>MGDDLLLKLLELLVEQARVSAEFARRQGDEKMLEEVARKAEEVARKAESIARKARKEGNLELALKALEILVRAAHVLAEIARERG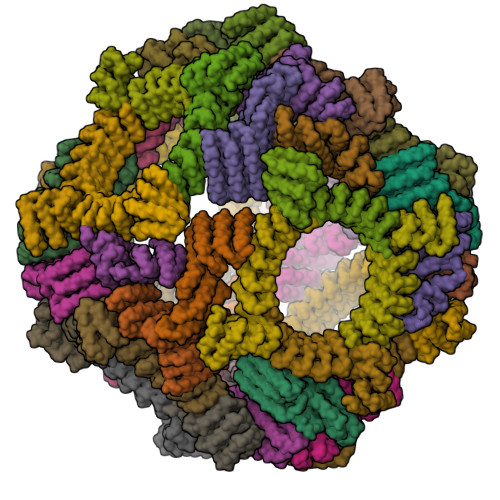NEELQKKAHKLAKEALRQVIEIAIRAIQEGNLELAIIALHISVRIAEVLLETRPDDREEIREQQAIFELLIAALEAAIRLEKLKEEGAPPEQIERVAEHGLERLKEIAKEISKEVDSPESKRIAYKIVAAAAEFLLKILAEGGATPEQLERVTEHALEVLKEVAKELADSPESGLAALAAIASLAKLGLEQLKEIGAPPEQQRRVTKAGIEAVREIYRYGRKLY[24x];>[24x]MGCDAIQAAAALGEAGISSNEILELLAAAAELGLDPDAIQAAAQLGEAGISSEEIKELLRAAHELGLDPDAIAAAADLGQAGVSPVEILALLIAASVLGLDPDAIQAAAALGEAGISAEEIIELLTAARDLGLDPDAIQAAAQLGEAGISSEEIKELLRAAHELGLDPDCIAAAADLGQAGISSSEITALLLAAAAIELAKRADDKDVREIVRDALELASRSTNDEVIRLALEAAVLAARSTDSDVLEIVKDALELAKQSTNEEVIKLALKAAVLAAKSTDEEVLEEVKEALRRAKESTDEEEIKEELRKAVEEAEGGSWLEHHHHHH>MHHHHHHASMDTARIAVVGAGVVGLSTAVCISKLVPRCSVTIISDKFTPDTTSDVAAGMLIPHTYPDTPIHTQKQWFRETFNHLFAIANSAEAGDAGVHLVSGWQIFQSTPTEEVPFWADVVLGFRKMTEAELKKFPQYVFGQAFTTLKYEGPAYLPWLEKRIKGSGGWTLTRRIEDLWELHPSFDIVVNCSGLGSRQLAGDSKIFPVRGQVLQVQAPWVEHFIRDGSGLTYIYPGTSHVTLGGTRQKGDWNLSPDAENSREILSR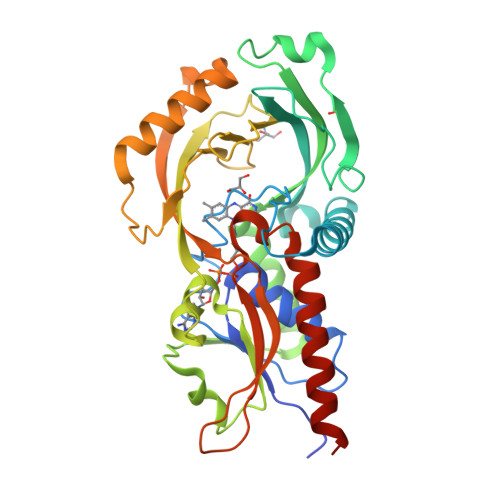CCALEPSLHGACNIREKVGLRPYRPGVRLQTELLARDGQRLPVVHHYGHGSGGISVHWGTALEAARLVSECVHALRTPIPKSNL[6x]> DNENVVNEYSSELEKHQLYIDETVNSNIPTNLRVLRSILENLRSKIQ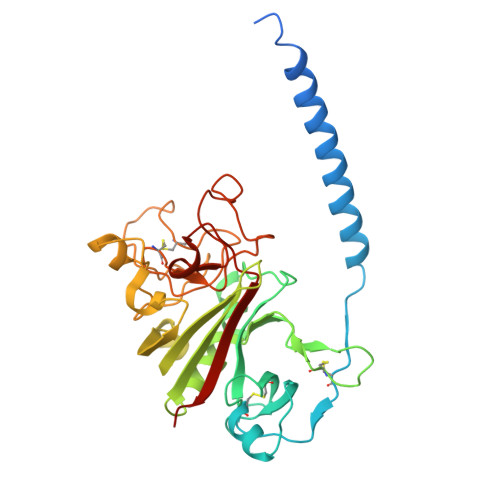KLESDVSAQMEYCRTPCTVSCNIPVVSGKECEEIIRKGGETSEMYLIQPDSSVKPYRVYCDMNTENGGWTVIQNRQDGSVDFGRKWDPYKQGFGNVATNTDGKNYCGLPGEYWLGNDKISQLTRMGPTELLIEMEDWKGDKVKAHYGGFTVQNEANKYQISVNKYRGTAGNALMDGASQLMGENRTMTIHNGMFFSTYDRDNDGWLTSDPRKQCSKEDGGGWWYNRCHAANPNGRYYWGGQYTWDMAKHGTADGVVWMNWKGSWYSMRKMSMKIRPFFPQQ> MAHHHHHHMAMEDNNKQIFNPKETKFLEEAEGVEALEWAKERTSKTEKALQAMQEYKQIKKEIETIFYDQRKTPYGVIRKGYVYNFWMDDKNPQGLWRRTLVDNYSKDKPNWEVLIDFDKLSKKIGKKVAYRGVSNCFQNPNRYLISMSFGGKDEMFFREWDLEKKDFVKNGFEPITNSGKLLEGKFTYPTWINKDTIIFNLVLHKNEITSSLYPNSLYIWKRGESIEKAKKLFEVPKEYIYVSAGKLLSDTISSSLIFISANKDFYNYDNYILDTKYKNLKLQKINMPSDATLQGSFKEYVFWLLRSDWKFKSHNIKAGSLVALHFTDLLKTESDKTSLKILFTPTANEVFNFISTTKDRVFLATYDNVVAKVVTFTLENEQWTKPVVLKLPYQNAIFGMSSYEEEEEALITIENSIVPPTIYLWVKTHELKIIRKALYSFDSENYVLEQKEATSFDGVKIPYFLVYKKGIKFDGKNPTLLEAYGGFQVINAPYFSRIKNEVWVKNAGVSVLANIRGGGEFGPEW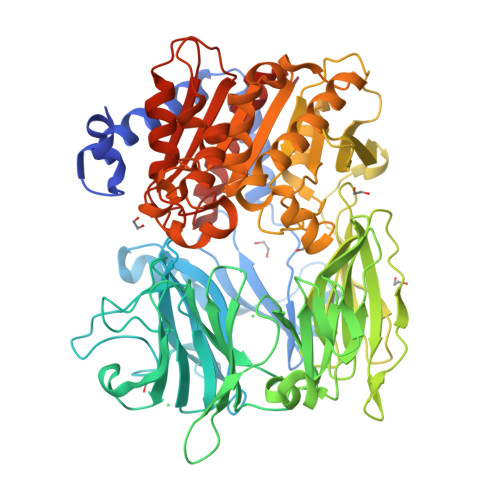HKSAQGIKRQTAFNDFFAVSEELIKQNITSPEYLGIKGGSNGGLLVSVAMTQRPELFGAVACEVPILDMIRYKEFGAGHSWVTEYGDPEIPNDLLHIKKYAPLENLSLTQKYPTVLITDSVLDQRVHPWHGRIFEYVLAQNPNTKTYFLESKDSGHGSGSDLKESANYFINLYTFFANALKLKIN[4-[(~{Z})-[(2~{R},5~{R})-5-(azanyloxymethyl)-3,6-bis(oxidanylidene)piperazin-2-yl]methoxyiminomethyl]-6-methyl-5-oxidanyl-pyridin-3-yl]methyl dihydrogen phosphate | C14 H20 N5 O9 P | 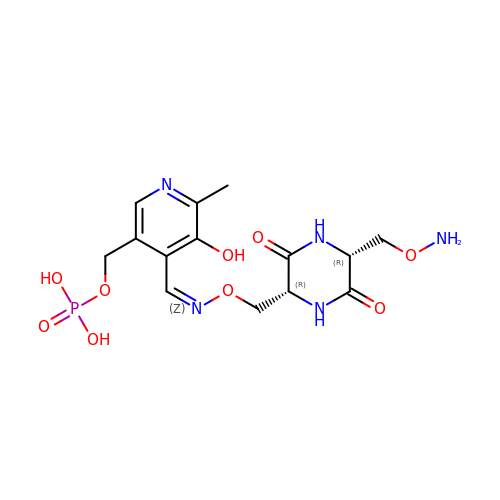HNXGFDLEQUEUAT-IZYPQUFVSA-N>[2x]MRMRHKPWADDFLAENADIAISNPADYKGKWNTVFGNDNPIHIEVGTGKGQFISGMAKQNPDINYIGIELFKSVIVTAVQKVKDSEAQNVKLLNIDADTLTDVFEPGEVKRVYLNFSDPWPK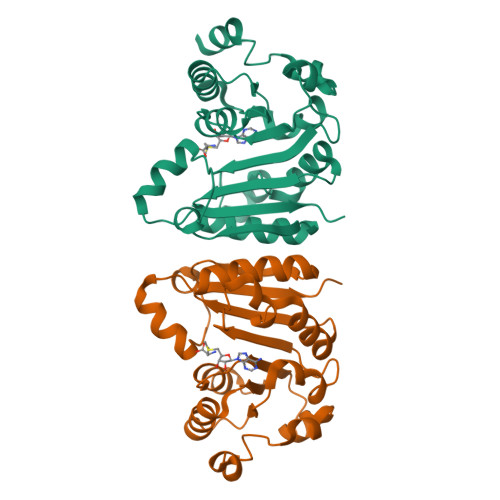KRHEKRRLTYSHFLKKYEEVMGKGGSIHFKTDNRGLFEYSLKSFSEYGLLLTYVSLDLHNSNLEGNIMTEYEEKFSALGQPIYRAEVEWRT>[4x]ASSSSKSSDSSAPKAYGYVYTADPETLDYLISSKNSTTVVTSNGIDGLFTNDNYGNLAPAVAEDWEVSKDGLTYTYKIRKGVKWFTSDGEEYAEVTAKDFVNGLKHAADKKSEAMYLAENSVKGLADYLSGTSTDFSTVGVKAVDDYTLQYTLNQPEPFWNSKLTYSIFWPLNEEFETSKGSDFAKPTDPTSLLYNGPFLLKGLTAKSSVEFVKNEQYWD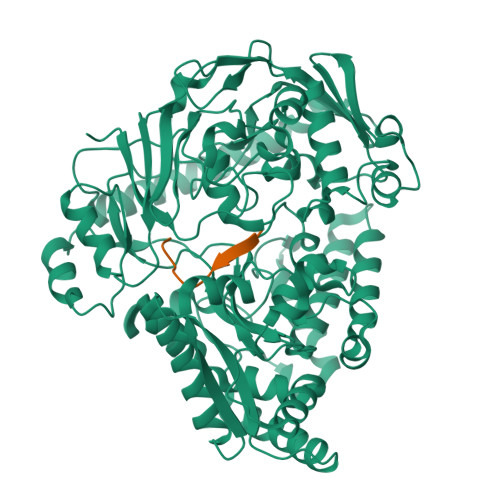KENVHLDTINLAYYDGSDQESLERNFTSGAYSYARLYPTSSNYSKVAEEYKDNIYYTQSGSGIAGLGVNIDRQSYNYTSKTTDSEKVATKKALLNKDFRQALNFALDRSAYSAQINGKDGAALAVRNLFVKPDFVSAGEKTFGDLVAAQLPAYGDEWKGVNLADGQDGLFNADKAKAEFAKAKKALEADGVQFPIHLDVPVDQASKNYISRIQSFKQSVETVLGVENVVVDIQQMTSDEFLNITYYAANASSEDWDVSGGVSWGPDYQDPSTYLDILKTTSSETTKTYLGFDNPNSPSVVQVGLKEYDKLVDEAARETSDLNVRYEKYAAAQAWLTDSSLFIPAMASSGAAPVLSRIVPFTGASAQTGSKGSDVYFKYLKSQDKVVTKEEYEKAREKWLKEKAESNEKAQKELASHVK;>[4x]AKTIKITQTR> GGPGRALCTPTFHGLSDGPYRRLKFSLKPIRHDYRDVLVSADLRKLAETAQELLRGKETKRRAFWEIFSKRVKASAHMLSPSLMALIAKSFDVHDRDTGIYVALATVLPEAVKRADGRSLLTLSDVFSRRLKRDSNPHLFSTLARQLPNALYQLTGKDVLRILSSLDAAGLADMLACRQ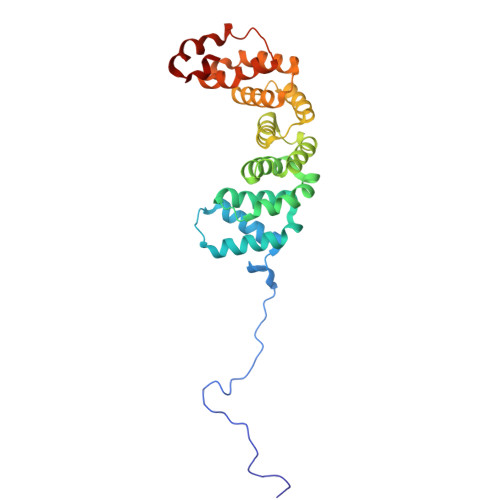VARKLLAELDELDSVDLADASAVFASQGYRNPELYSALARRAVDVKDSFDAPTVFRLLSGFSQNAVACDELLESFSTLLVSSKDQFTQHER>[4x]MLVVGSELQSDAQQLSAEAPRHGELQYLRQVEHILRCGFKKEDRTGTGTLSVFGMQARYSLRDEFPLLTTKRVFWKGVLEELLWFIKGSTNAKELSSKGVRIWDANGSRDFLDSLGFSARQEGDLGPVYGFQWRHFGAEYKDMDSDYSGQGVDQLQKVIDTIKTNPDDRRIIMCAWNPKDLPLMALPPCHALCQFYVVNGELSCQLYQRSGDMGLGVPFNIASYALLTYMIAHITGLQPGDFVHTLGDAHIYLNHIEPLKIQLQREPRPFPKLKILRKVETIDDFKVEDFQIEGYNPHPTIKMEMAV

Thymidylate synthase (TS; EC 2.1.1.45), a target enzyme in antitumor chemotherapy, catalyzes the N(5,10)-methylenetetrahydrofolate- (mTHF-) dependent C(5)-methylation of deoxyuridylate (dUMP), leading to the formation of thymidylate (dTMP), a nucleotide required for DNA biosynthesis. The enzyme, being a homodimer, is strongly conserved among the prokaryotic and eukaryotic species, from bacteria to mammals. A feature distinguishing mammalian from bacterial TS enzymes is N-terminal extension by some 27 amino acid residues, present in the former but absent in the latter enzymes. However, that protein segment is usually disordered and thus absent in the crystal structures of a mammalian TS.

The present paper reports the first structure of mammalian TS—the tertiary complex of mouse TS (mTS) with dUMP and the strong antifolate inhibitor and anticancer drug, Raltitrexed—with a clearly defined segment of 13 N-terminal amino acids. The crystal structure of mouse thymidylate synthase (mTS) in complex with dUMP and Raltitrexed comprises two homodimers, AB and CD, consisting of chains A, B, C, and D, represented by continuous and (overall) well-defined electron densities for amino acids 21–307, 20–307, 21–302, and 21–304, respectively. The ligands, dUMP and Raltitrexed, are described by clear electron densities in all subunits. Unexpectedly, an N-terminal segment consisting of residues 1–13, usually disordered in mammalian thymidylate synthases, is clearly visible in all subunits, even though the following segment 14–20 (14–19 in chain B) is not visible on the electron density maps and has not been included in the final model. The segment was stable enough to show up unambiguously on the electron density maps, probably owing to crystal packing, rather than intramolecular interactions. The subunit active sites are similar within each dimer but significantly different between the two dimers AB and CD, with the latter being related to the degree of the closure of a given active site. Moreover, considering noticeable electron densities between mTS Cys189 γS and dUMP C6 in the subunits A and B, including continuous electron density at 1.8σ in the latter subunit, the presence of the γS-C6 covalent bond in some fraction of the population of mTS-dUMP-Raltitrexed molecules may be expected. In addition, in accord with more closed conformation of the dimer AB than CD, the C-terminal segment that contributes to the active site closing and enzyme catalysis is described by a well-defined electron density throughout the segment in the former, in contrast to a weaker electron density, resulting in the lack of a few most terminal residues in the latter. Altogether, these results show Raltitrexed binding to influence the present structure in an asymmetric manner, changing the conformation of one protein dimer (AB) more than the other (CD).>[2x]MRALLLSGCLALVLLTQQAAAQTLLVVGDSISAALGLD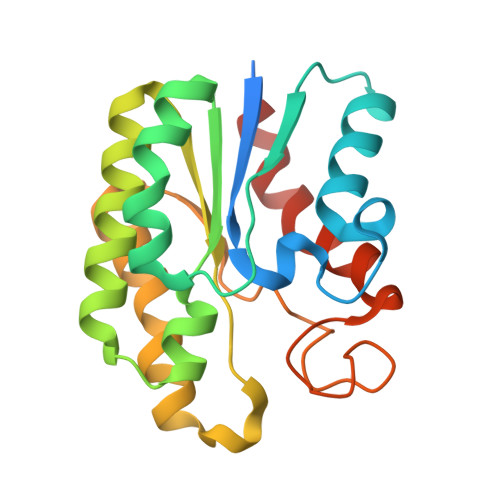TSQGWVALLQKRLADEGYDYRVVNASISGDTSAGGLARLPALLAEEKPALVVIELGGNDGLRGMAPAQLQQNLASMAQKARAEGAKVLLLGIQLPPNYGPRYIEAFSRVYGAVAAQEKTALVPFFLEGVGGVQGMMQADGIHPALAAQPRLLENVWPTLKPLLHHHHHH>[2x]AMKNKVQLITYADRLGDGTIKSMTDILRTRFDGVYDGVHILPFFTPFDGADAGFDPIDHTKVDERLGSWDDVAELSKTHNIMV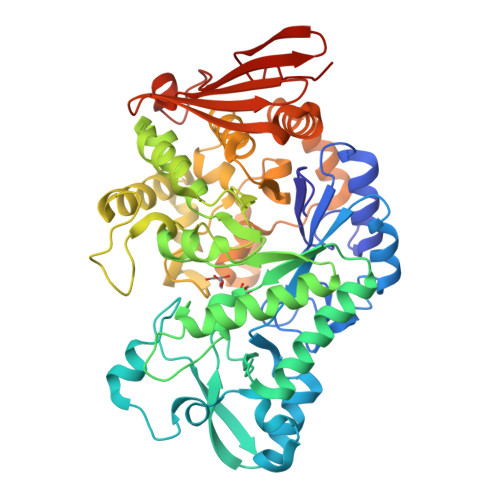DAIVNHMSWESKQFQDVLAKGEESEYYPMFLTMSSVFPNGATEEDLAGIYRPRPGLPFTHYKFAGKTRLVWVSFTPQQVDIDTDSDKGWEYLMSIFDQMAASHVSYIRLDAVGYGAKEAGTSCFMTPKTFKLISRLREEGVKRGLEILIEVHSYYKKQVEIASKVDRVYDFALPPLLLHALSTGHVEPVAHWTDIRPNNAVTVLDTHDGIGVIDIGSDQLDRSLKGLVPDEDVDNLVNTIHANTHGESQAATGAAASNLDLYFVNSTYYSALGCNDQHYIAARAVQFFLPGVPQVYYVGALAGKNDMELLRKTNNGRDINRHYYSTAEIDENLKRPVVKALNALAKFRNELDAFDGTFSYTTDDDTSISFTWRGETSQATLTFEPKRGLGVDNTTPVAMLEWEDSAGDHRSDDLIANPPVVAA> DPDVDECQLMPNACQNGGTCHNSHGGYNCVCVNGWTGEDCSENIDDCASAACFQGATCHDRVASFYCECPHGRTGLLCHLNDACISNPCNEGSNCDTNPVNGKAICTCPSGYTGPACSQDVDECALGANPCEHAGKCLNTLGSFECQCLQGYTGPRCEIDVNECISNPCQNDATCLDQIGEFQCICMPGYEGVYCESGRLEVLFQ;> ADPRLGQFELEILSMQNVNGELQNGNCCGGARNPGDRKCTGDECNTYFKVCLKEYQSRVRAGGPCSFGSGSTPVIGGNTFNLKASRGNDRNRIVLPFSFAWPRSYTLLVEAWDSSNDTIQPDSIIEKASHSGMINPSRQW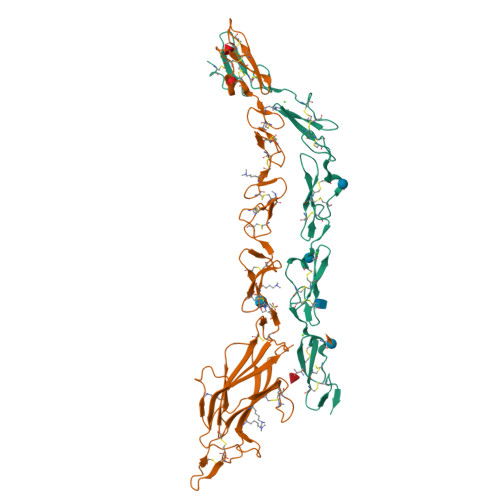QTLKQNTGIAHFEYRIRVTCDDHYYGFGCNKFCRPRDDFFGHYACDQNGNKTCMEGWMGPECNKAICRQGCSPKHGSCKLPGDCRCQYGWQGLYCDKCIPHPGCVHGTCNEPWQCLCETNWGGQLCDKDLNYCGTHQPCLNRGTCSNTGPDKYQCSCPEGYSGPNCEAAAHHHHHHHH Finding a correct substrate is especially difficult for the Escherichia coli Nudix hydrolase RppH, which triggers 5′-end-dependent RNA degradation by removing orthophosphate from the 5′-diphosphorylated transcripts. In Escherichia coli and probably many other bacteria, RppH converts diphosphorylated 5′ ends of transcripts into monophosphorylated ends that accelerate subsequent cleavage by the 5′-monophosphate-stimulated endonuclease RNase E. Escherichia coli RppH can also remove pyrophosphate from triphosphorylated RNA with lower efficiency. Here we show that RppH binds and slowly hydrolyzes NTPs, NDPs and (p)ppGpp, which each resemble the 5′-end of RNA. A series of X-ray crystal structures of RppH-nucleotide complexes, trapped in conformations either compatible or incompatible with hydrolysis, explain the low reaction rates of mononucleotides and suggest two distinct mechanisms for their hydrolysis.

To understand how nucleotides inhibit the reaction of RppH with the RNA substrates, we determined 1.6–1.9 Å crystal structures of RppH bound to triphosphorylated nucleosides and/or their non-hydrolysable analogs, ppcpNs, which contain a methylene moiety instead of a bridging oxygen atom between α- and β-phosphates. Neither structure contains Mg2+ cations since their addition to the crystallization solution resulted in the loss of electron density map for nucleotides, even for non-hydrolysable substrate analogs and at pH values unfavorable for catalysis. In the absence of Mg2+, the map for nucleotides was of high quality although the occupancy of nucleotides was refined to lower than 100% in some cases. In all of the structures, the position of the nucleobases is nearly invariant, while the conformations of the sugar–phosphate moieties have small differences. All of the nucleobases bind in the protein cleft where we previously observed specific binding of guanosine at the second position of an RNA ligand. In this cleft, the nucleobase is sandwiched between the guanidinium group of R27 and a hydrophobic pedestal formed by V137 and F139. Pyrimidines are locked in place by a hydrogen bond with S32, while purines are likely held by stronger cation–π interactions with R27. The sugar–phosphate moiety is oriented toward the catalytic site and forms several hydrogen bonds involving R27, Y77, Q95 and K140 in all of the structures. Thus, the NTP-bound structures demonstrate that NTPs interact with RppH in the same site where the second nucleotide of RNA binds RppH. In this position, NTPs can compete with RNA for RppH binding and inhibit the reaction of RNA substrates.

> SMIDDDGYRPNVGIVICNRQGQVMWARRFGQHSWQFPQGGINPGESAEQAMYRELFEEVGLSRKDVRILASTRNWLRYKLPKRLVRWDTKPVCIGQKQKWFLLQLVSGDAEINMQTSSTPEFDGWRWVSYWYPVRQVVSFKRDVYRRVMKEFASVVMSLAA>MEQAMRERSELARKGIARAKSVVALAYAGGVLFVAENPSRSLQKISELYDRVGFAAAGKFNEFDNLRRGGIQFADTRGYAYDRRDVTGRQLANVYAQTLGTIFTEQAKPYEVELCVAEVAHYGETKRPELYRITYDGSIADEPHFVVMGGTTEPIANALKESYAENASLTDALRIAVAALRAGSADTSGGDQPTLGVASLEVAVLDANRPRRAFRRITGSALQALLVDQESPQSDGESSG[28x];>XTIVALKYPGGVVMAGDRRSTQGNMISGRDVRKVYITDDYTATGIAGTA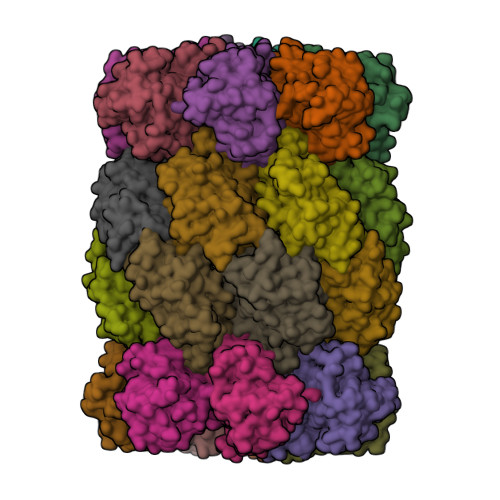AVAVEFARLYAVELEHYEKLEGVPLTFAGKINRLAIMVRGNLAAAMQGLLALPLLAGYDIHASDPQSAGRIVSFDAAGGWNIEEEGYQAVGSGSLFAKSSMKKLYSQVTDGDSGLRVAVEALYDAADDDSATGGPDLVRGIFPTAVIIDADGAVDVPESRIAELARAIIESRSGADTFGSDGGEKHHHHHH[28x]>[2x]TDTTLPPDDSLDRIEPVDIEQEMQRSYIDYAMSVIVGRALPEVRDGLKPVHRRVLYAMFDSGFRPDRSHAKSARSVAETMGNYHPHGDSSIYDSLVRMAQPWSLRYPLVDGQGNFGSPGNDPPAAMRYTEARLTPLAMEMLREIDEETVDFIPNYDGRVQEPTVLPSRFPNLLANGSGGIAVGMATNIPPHNLRELADAVFWALENHDADEEETLAAVMGRVKGPDFPTAGLIVGSQGTADAYKTGRGSIRMRGVVEVEEDSRGRTSLVITELPYQVNHDNFITSIAEQVRDGKLAGISNIEDQSSDRVGLRIVIEIKRDAVAKVVINNLYKHTQLQTSFGANMLAIVDGVPRTLRLDQLIRYYVDHQLDVIVRRTTYRLRKANERAHILRGLVKALDALDEVIALIRASETVDIARAGLIELLDIDEIQAQAILDMQLRRLAALERQRIIDDLAKIEAEIADLEDILAKPERQRGIVRDELAEIVDRHGDDRR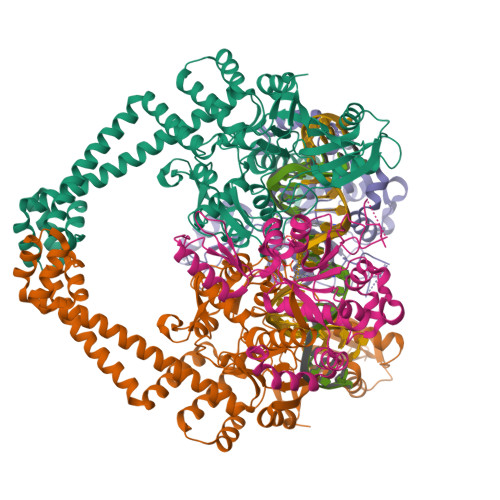TRIIAIGSG;>[2x]SNALVRRKSATDIGGLPGKLADCRSTDPRKSELYVVEGDSAGGSAKSGRDSMFQAILPLRGKIINVEKARIDRVLKNTEVQAIITALGTGIHDEFDIGKLRYHKIVLMADADVDGQHISTLLLTLLFRFMRPLIENGHVFLAQPPLYKLKWQRSDPEFAYSDRERDGLLEAGLKAGKKINKEDGIQRYKGLGEMDAKELWETTMDPSVRVLRQVTLDDAAAADELFSILMGEDVDARRSFITRNAKDVRFLDV>[2x]MASGSASSAQTPGLMSWLPPSNQLSPEARSVLDRMDAAKAPEFNGDLVRQRAFYQQFNDDRLVEMRRVFRTRERHETLNAVHVQVVEPADGVSARNRDRVLINVHGGAFMWGAGSGALVEAIPIAATMGVSVVTVDYRLAPENRYPAASEDVTAVYRALLERYPAANIGIFGSSAGGVITAQAVTWIRREGLPRPGAIGTLCGTGAPYSGDSPYLAGVVPVGPGVKAPPLPGLLPTA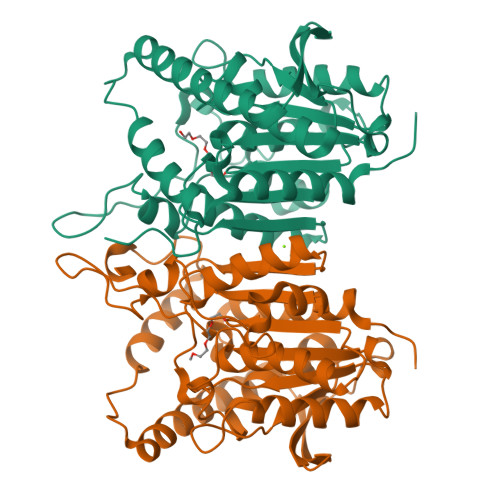YMEGVGADDARAYPLTSDAETVFMPPTLLLAGGRDFAVSALSLAHRRLARAGVDSELHLFDGLPHAFFVWPDMPESLEAYALIAGFFDSRLGLTPSSSIPTPRSPSLEHHHHHH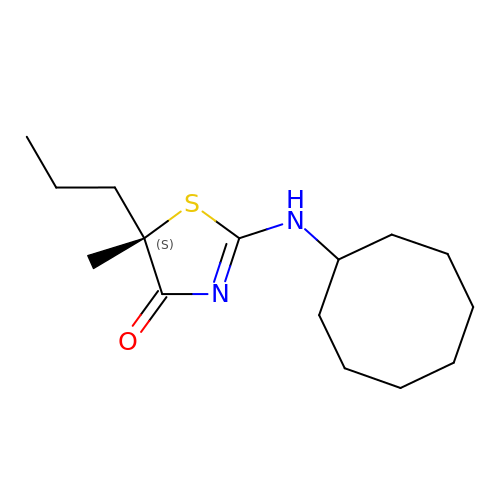(5S)-2-(cyclooctylamino)-5-methyl-5-propyl-1,3-thiazol-4(5H)-one | C15 H26 N2 O S | SBTHYUAUBLEDJY-HNNXBMFYSA-N> SNAEERLKMSTTTSTQDSGLLKVLLPPFEKKNNVKVDVIAVGTGQALKLGEAGDVDVVFVHARKLEDKFVADGFGVNRKDVMYNDFVIVGPKNDPAGIAKAKTAAEALKLLATKGATFISRGDKSGTHTKELD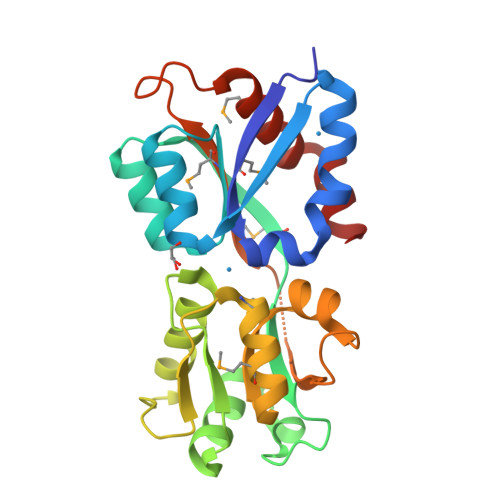LWKSAGVDPKGNWYVEAGQGMGPVITMATERRAYTLTDRGTYNAFKGAKTDLVILFQGEKGLFNPYGIMAVNPKKFPHVKYDLAMKLIDYVTGPEGLKIISDY> GPGSELPQMVQQLNSPDQQELQSALRKLSQIASGGNEQIQAVIDAGALPALVQLLSSPNEQILQEALWALSNIASGGNEQIQAVIDAGALPALVQLLSSPNEQILQEALWALSNIASGGNEQIQAVIDAGALPALVQLLSSPNEQILQEALWALSNIASGGNEQIQAVIDAGALPALVQLLSSPNEQILQEALWALSNIASGGNEQIQAVIDAGALPALVQLLSSPNEQILQEALWALSNIASGGNEQKQAVKEAG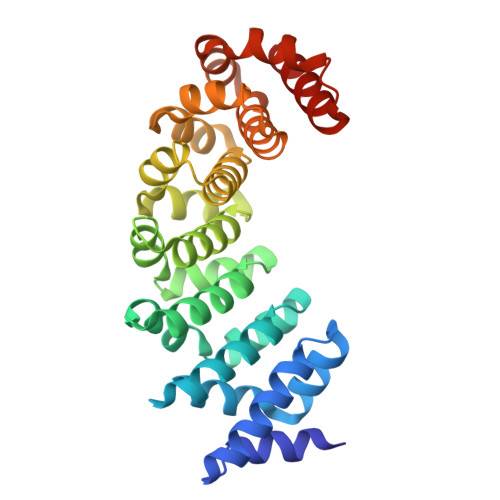ALEKLEQLQSHENEKIQKEAQEALEKLQSH>[3x]GSHMNIITVTLNMEKYNFLGISIVGQSNERGDGGIYI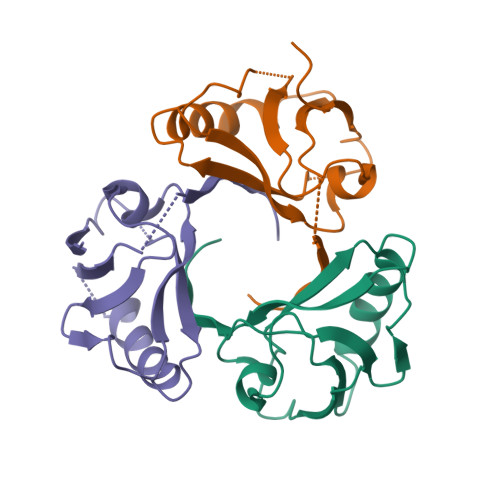GSIMKGGAVAADGRIEPGDMLLQVNDMNFENMSNDDAVRVLRDIVHKPGPIVLTVAKSGGGGEIVLWSDIP> GPLGSAPVRSLNCTLRDSQQKSLVMSGPYELKALHLQGQDMEQQVVFSMSFVQGEESNDKIPVALGLKEKNLYLSCVLKDDKPTLQLESVDPKNYPKKKMEKRFVFNKIEINNKLEFESAQFPNWYISTSQAENMP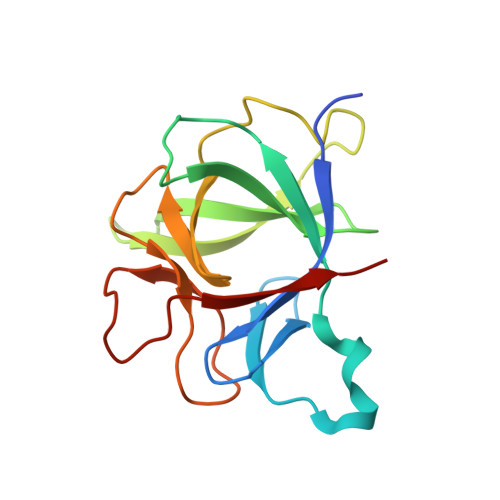VFLGGTKGGQDITDFTMQFVSS> MKKGHHHHHHGSERTGTQPLGVQGLTEEQRMMIRELMDAQMKTFDTTFSHFKNFRLPGVLSSGCELPESLQAPSREEAAKWSQVRKDLCSLKVSLQLRGEDGSVWNYKPPADSGGKEIFSLLPHMADMSTYMFKGIISFAKVISYFRDLPIEDQISLLKGAAFELCQLRFNTVFNAETGTWECGRLSYCLEDTAGGFQQLLLEPMLKF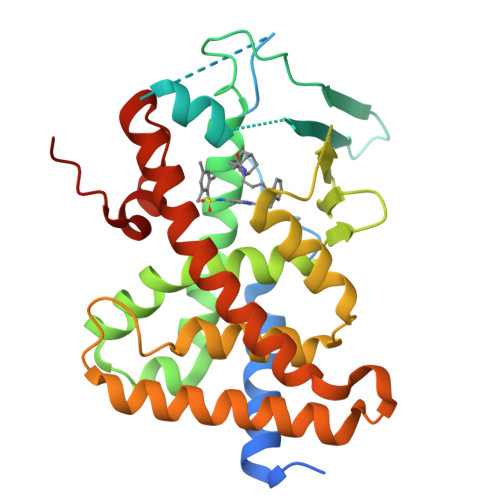HYMLKKLQLHEEEYVLMQAISLFSPDRPGVLQHRVVDQLQEQFAITLKSYIECNRPQPAHRFLFLKIMAMLTELRSINAQHTQRLLRIQDIHPFATPLMQELFGITGSLVPR> MQDAITSVINSSDVQGKYLDNAALEKLKGYFATGELRV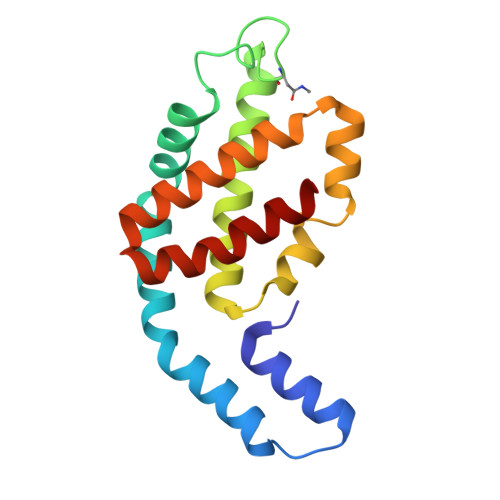RAATTISANAAAIVKEAVAKSLLYSDITRPGGNMYTTRRYAACIRDLDYYLRYATYAMLAGDPSILDERVLNGLKETYNSLGVPVGATVQAIQAIKEVTASLVGPDAGKEMGVYFDYICSGLS>[3x]MSNEVEQKKNIKTIND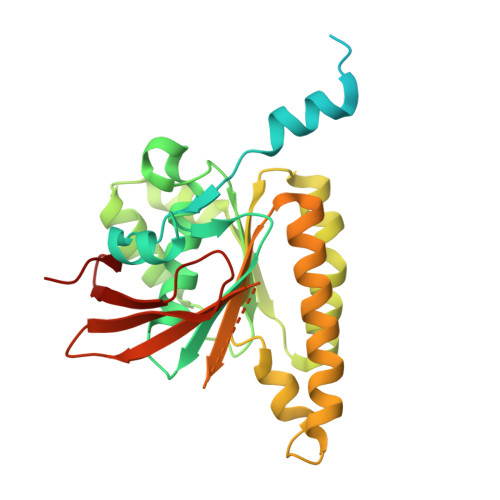LPGISQTVINKLIEAGYSSLETLAVASPQDLSVAAGIPLSTAQKIIKEARDALDIRFKTALEVKKERMNVKKISTGSQALDGLLAGGIETRTMTEFFGEFGSGKTQLCHQLSVNVQLPPEKGGLSGKAVYIDTEGTFRWERIENMAKALGLDIDNVMNNIYYIRAINTDHQIAIVDDLQELVSKDPSIKLIVVDSVTSHFRAEYPGRENLAVRQQKLNKHLHQLTRLAEVYDIAVIITNQVMARPDMFYGDPTVAVGGHTLYHVPGIRIQLKKSRGNRRIARVVDAPHLPEGEVVFALTEEGIRDAEE> GMSDVAETLDPLRLPLQGERLIEASAGTGKTFTIAALYLRLLLGLGGSAAFPRPLTVEELLVVTFTEAATAELRGRIRSNIHELRIACLRETTDNPLYERLLEEIDDKAQAAQWLLLAERQMDEAAVFTIHGFCQRMLNLNAFESGMLFEQQLIEDESLLRYQACADFWRRHCYPLPREIAQVVFETWKGPQALLRDINRYLQGEAPVIKAPPPDDETLASRHAQIVARIDTVKQQWRDAVGELDALIESSGIDRRKFNRSNQAKWIDKISAWAEEETNSYQLPESLEKFSQRFLEDRTKAGGETPRHPLFEAIDQLLAEPLSIRDLVITRALAEIRETVAREKRRRGELGFDDMLSRLDSALRSESGEVLAAAIRTRFPVAMIDEFQDTDPQQYRIFRRIWHHQPETALLLIGDPKQAIYAFRGADIFTYMKARSEVHAHYTLDTNWRSAPGMVNSVNKLFSQTDDAFMFREIPFIPVKSAGKNQALRFVFKGETQPAMKMWLMEGESCGVGDYQSTMAQVCAAQIRDWLQAGQRGEALLMNGDDARPVRASDISVLVRSRQEAAQVRDALTLLEIPSVYLSNRDSVFETLEAQEMLWLLQAVMTPERENTLRSALATSMMGLNALDIETLNNDEHAWDVVVEEFDGYRQIWRKRGVMPMLRALMSARNIAENLLATAGGERRLTDILHISELLQEAGTQLESEHALVRWLSQHILEPDSNASSQQMRLESDKHLVQIVTIHKSKGLEYPLVWLPFITNFRVQEQAFYHDRHSFEAVLDLNAAPESVDLAEAERLAEDLRLLYVALTRSVWHCSLGVAPLVRRRGDKKGDTDVHQSALGRLLQKGEPQDAAGLRTCIEALCDDDIAWQTAQTGDNQPWQVNDVSTAELNAKTLQRLPGDNWRVTSYSGLQQRXXXXXXXXXXXXXXXXXXXXXXXXXPTLTPHQFPRGASPGTFLHSLFEDLDFTQPVDPNWVREKLELGGFESQWEPVLTEWITAVLQAPLNETGVSLSQLSARNKQVEMEFYLPISEPLIASQLDTLIRQFDPLSAGCPPLEFMQVRGMLKG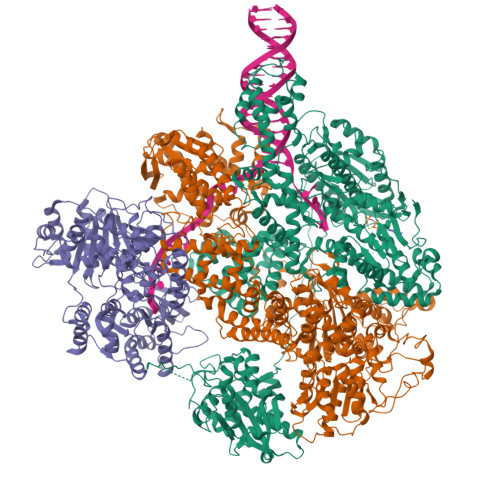FIDLVFRHEGRYYLLAYKSNWLGEDSSAYTQQAMAAAMQAHRYDLQYQLYTLALHRYLRHRIADYDYEHHFGGVIYLFLRGVDKEHPQQGIYTTRPNAGLIALMDEMFAGMTLEEA;> MLRVYHSNRLDVLEALMEFIVERERLDDPFEPEMILVQSTGMAQWLQMTLSQKFGIAANIDFPLPASFIWDMFVRVLPEIPKESAFNKQSMSWKLMTLLPQLLEREDFTLLRHYLTDDSDKRKLFQLSSKAADLFDQYLVYRPDWLAQWETGHLVEGLGEAQAWQAPLWKALVEYTHQLGQPRWHRANLYQRFIETLESATTCPPGLPSRVFICGISALPPVYLQALQALGKHIEIHLLFTNPCRYYWGDIKDPAYLAKLLTRQRRHSFEDRELPLFRDSENAGQLFNSDGEQDVGNPLLASWGKLGRDYIYLLSDLESSQELDAFVDVTPDNLLHNIQSDILELENRAVAGVNIEEFSRSDNKRPLDPLDSSITFHVCHSPQREVEVLHDRLLAMLEEDPTLTPRDIIVMVADIDSYSPFIQAVFGSAPADRYLPYAISDRRARQSHPVLEAFISLLSLPDSRFVSEDVLALLDVPVLAARFDITEEGLRYLRQWVNESGIRWGIDDDNVRELELPATGQHTWRFGLTRMLLGYAMESAQGEWQSVLPYDESSGLIAELVGHLASLLMQLNIWRRGLAQERPLEEWLPVCRDMLNAFFLPDAETEAAMTLIEQQWQAIIAEGLGAQYGDAVPLSLLRDELAQRLDQERISQRFLAGPVNICTLMPMRSIPFKVVCLLGMNDGVYPRQLAPLGFDLMSQKPKRGDRSRRDDDRYLFLEALISAQQKLYISYIGRSIQDNSERFPSVLVQELIDYIGQSHYLPGDEALNCDESEARVKAHLTCLHTRMPFDPQNYQPGERQSYAREWLPAASQAGKAHSEFVQPLPFTLPETVPLETLQRFWAHPVRAFFQMRLQVNFRTEDSEIPDTEPFILEGLSRYQINQQLLNALVEQDDAERLFRRFRAAGDLPYGAFGEIFWETQCQEMQQLADRVIACRQPGQSMEIDLACNGVQITGWLPQVQPDGLLRWRPSLLSVAQGMQLWLEHLVYCASGGNGESRLFLRKDGEWRFPPLAAEQALHYLSQLIEGYREGMSAPLLVLPESGGAWLKTCYDAQNDAMLDDDSTLQKARTKFLQAYEGNMMVRGEGDDIWYQRLWRQLTPETMEAIVEQSQRFLLPLFRFNQS;> MGKLQKQLLEAVEHKQLRPLDVQFALTVAGDEHPAVTLAAALLSHDAGEGHVCLPLSRLENNEASHPLLATCVSEIGELQNWEECLLASQAVSRGDEPTPMILCGDRLYLNRMWCNERTVARFFNEVNHAIEVDEALLAQTLDKLFPVSDEINWQKVAAAVALTRRISVISGGPGTGKTTTVAKLLAALIQMADGERCRIRLAAPTGKAAARLTESLGKALRQLPLTDEQKKRIPEDASTLHRLLGAQPGSQRLRHHAGNPLHLDVLVVDEASMIDLPMMSRLIDALPDHARVIFLGDRDQLASVEAGAVLGDICAYANAGFTAERARQLSRLTGTHVPAGTGTEAASLRDSLCLLQKSYRFGSDSGIGQLAAAINRGDKTAVKTVFQQDFTDIEKRLLQSGEDYIAMLEEALAGYGRYLDLLQARAEPDLIIQAFNEYQLLCALREGPFGVAGLNERIEQFMQQKRKIHRHPHSRWYEGRPVMIARNDSALGLFNGDIGIALDRGQGTRVWFAMPDGNIKSVQPSRLPEHETTWAMTVHKSQGSEFDHAALILPSQRTPVVTRELVYTAVTRARRRLSLYADERILSAAIATRTERRSGLAALFSSRE Perforin-2 (MPEG1) is thought to enable the killing of invading microbes engulfed by macrophages and other phagocytes, forming pores in their membranes. Perforin-2 (PFN2) has recently been identified as a novel and critically important component of innate immunity conserved throughout the animal kingdom and evolutionarily close to the last common ancestor of the MAC and perforin-1 (7, 10). Because of the presence of a canonical MAC-perforin (MACPF) domain, PFN2 has been proposed to form functional pores in bacterial membranes, leading to bacterial death and control of infection. However, unlike MAC components and perforin-1, PFN2 is initially synthesized as a type I transmembrane protein and found associated with the membranes of intracellular vesicles in which its large ectodomain (consisting mainly of the MACPF domain and a unique P2 domain characteristic of PFN2) projects into the lumen.

A complete (180°) reconfiguration of the MACPF and membrane-binding P2 domains triggered by acidification then results in pore formation. We were able to construct a model of the pore fitted to its cryo-EM density guided by the distinctive features of each PFN2 domain and their connectivity and the conserved two glycans visible in both structures. We were unable to resolve the CTT domain due to the absence of density for the CTT in the PFN2 pore map, suggesting that it may have become intrinsically disordered on pore formation. Our structure confirms the rotation between the MACPF and P2 domains by 180° and reveals other conformational changes accompanying membrane insertion including the deployment of TMH1 and TMH2 to generate a 64-stranded β-barrel. In the pore form, the MACPF domain has rotated with respect to the P2 domain by ~180° when viewed from the side and by ~90° when viewed from above (looking down toward the membrane surface) compared to its position in the pre-pore, resulting in a compound screw rotation. The pore-forming oligomer structure is entirely consistent with the pores imaged directly on liposome membranes and is 206 Å in diameter and 140 Å tall from the top of the MACPF domain to the tip of the β-barrel. Side views of membrane-inserted pores were very different from those of pre-pores, with obvious transmembrane channels and standing significantly taller than the pre-pore form (110 Å compared to 85 Å). Upon exposure to a low pH shock, the PFN2 pre-pore rings began to form pores after 14 s and all ~70 being imaged transited to the pore state within 3 s. The resulting structures were higher (raised by ~4 nm) compared to the pre-pore state, in agreement with the pores imaged by negative-stain electron microscopy. Overall, these results show that acidic pH triggers pre-pore–to–pore transformation, which is achieved by a 180° rotation of the MACPF and P2 domains with respect to each other so that membrane insertion can occur.

>ETGDKPLGETGTTGFQICKNALKLPVLEVLPGGGWDNLRNVDMGRVMDLTYTNCKTTEDGQYIIPDEVYTIPQKESNLEMNSEVLESWMNYQSTTSLSINTELALFSRVNGKFSTEFQRMKTLQVKDQAVTTRVQVRNRIYTVKTTPTSELSLGFTKALMDICDQLEKNQTKMATYLAELLILNYGTHVITSVDAGAALVQEDHVRSSFLLDNQNSQNTVTASAGIAFLNIVNFKVETDYISQTSLTKDYLSNRTNSRVQSFGGVPFYPGITLETWQKGITNHLVAIDRAGLPLHFFIKPDKLPGLPGPLVKKLSKTVETAVRHYYTFNTHPGCTNVDSPNFNFQANMDDDSCDAKVTNFTFGGVYQECTELSGDVLCQNLEQKNLLTGDFSCPPGYSPVHLLSQTHEEGYSRLECKKKCTLKIFCKTVCEDVFRVAKAEFRAYWCVAAGQVPDNSGLLFGGVFTDKTINPMTNAQSCPAGYIPLNLFESLKVCVSLDYELGFKFSVPFGGFFSCIMGNPLVNSDTAKDVRAPSLKKCPGGFSQHLAVISDGCQVSYCVKAGIFTGGSLLPVRLPPYTKPPLMSQVATNTVIVTNSETARSWIKDPQTNQWKLGEPLELRRAMTVIHGDSNGMSGGGTETSQVAPA[16x]> STDNAETGVIEAGNTDTDFSGELAAPGSNHTNVKFLFDRSRLLNVIKVLEKDAVFPRPFPTQEGAQQDDGYFCLLTPRPTVASRPATRFGLYANPSGSGVLANTSLDFNFYSLACFTYFRSDLEVTVVSLEPDLEFAVGWFPSGSEYQASSFVYDQLHVPFHFTGRTPRAFASKGGKVSFVLPWNSVSSVLPVRWGGASKLSSATRGLPAHADWGTIYAFVPRPNEKKSTAVKHVAVYIRYKNARAWCPSMLPFRSYK;> GPIPTAPRENSLMFLSTLPDDTVPAYGNVRTPPVNYLPGEITDLLQLARIPTLMAFERVPEPVPASDTYVPYVAVPTQFDDRPLISFPITLSDPVYQNTLVGAISSNFANYRGCIQITLTFCGPMMARGKFLLSYSPPNGTQPQTLSEAMQCTYSIWDIGLNSSWTFVVPYISPSDYRETRAITNSVYSADGWFSLHKLTKITLPPDCPQSPCILFFASAGEDYTLRLPVDCNPSYVF;> DRVTTQTAGNTAINTQSSLGVLCAYVEDPTKSDPPSSSTDQPTTTFTAIDRWYTGRLNSWTKAVKTFSFQAVPLPGAFLSRQGGLNGGAFTATLHRHFLMKCGWQVQVQCNLTQFHQGALLVAMVPETTLDVKPDGKAKSLQELNEEQWVEMSDDYRTGKNMPFQSLGTYYRPPNWTWGPNFINPYQVTVFPHQILNARTSTSVDINVPYIGETPTQSSETQNSWTLLVMVLVPLDYKEGATTDPEITFSVRPTSPYFNGLRNRYTAG;> RGNNGNMTFNYYANTYQNSVDFSTSSSASGAGPGNSRGGLAGLLTNFSGILNPLGYLK

Seneca Valley virus (SVV) is an oncolytic picornavirus that selectively targets cancer cells by recognizing Tumor endothelial marker 8 (TEM8) as the host receptor. SVV has a typical picornavirus capsid with four capsid proteins; VP1, VP2, and VP3 are characterized by a single jelly roll fold, where eight beta-strands form a barrel-like structure that is distributed at the exterior of the virus, while VP4 is located on the interior of the capsid. The structural architecture consists of four capsid proteins forming a protomer, 5 protomers forming a pentamer, and 12 pentamers assembling into a pseudo T=3 capsid, approximately ~32 nm in diameter. We used cryo-electron microscopy to investigate SVV under acidic conditions and in complex with TEM8 at physiological pH, identifying multiple uncoating intermediates.

We used cryo-EM to image SVV particles after incubation at pH 5 and 37°C with purified TEM8 to explore the structural behavior of SVV. For both physiological and acidic conditions, the A-particles were resolved to 3.4 Å, while for the ER-particles, the resolutions were 6.4 and 4.3 Å, respectively. The A-particles obtained in both conditions are expanded by ~5% in diameter compared to the F-particle. This expansion results in reduced capsid protein contacts compared to the F-particle. Inter-pentamer contacts are reduced by 34% and 22% under acidic and physiological conditions, respectively. For the A-particle[P], additional disordered regions without interpretable density include VP1 (G13, S20, and S28), VP2 (D12), and VP3 (E61-S66), while for the A-particle[C], these include VP3 (P60-D67). On the capsid exterior, the A-particle[P] had the following partially ordered regions: the VP1 HI loop (S229), VP1 BC loop (A65), VP1 Loop II (G97), and VP2 residues V59 and D67, while the A-particle[C] exhibited similar behavior showing partially ordered regions: VP1 HI loop (T230) and VP1 Loop II (P95-G97). For the A-particle[C], the disordered regions were on the VP1 N-terminus (E11-S28) and VP4 residues G63 to N66. Density corresponding to TEM8 was not visible on the SVV A- and ER-particles under acidic conditions, suggesting that at low pH, the virus potentially loses the affinity for the receptor or binds transiently. In the SVV A-particle, its genome is reorganized and lacks defined capsid-RNA interactions with the inner capsid surface, likely contributing to the flexibility of the VP1 N-terminus, which is consequently poorly resolved.>KMAKDSKAPVVEIFDERDGCTSAGSTGKASDAGEKGLLVKVSMQKVGYNAIMAKSVAASYMNK[2x];>[2x]MLDAFSKVITSADGKAAYVGGADLQALKKFVSDGNKRMDAVNAIVSNASCIVSDAVSGMVCENPSLIAPNGGVYSNRKMAACLRDAEIILRYVSYSLLSGDSSVLEDRCLNGLKETYSSLGVPAAGNARAVAIM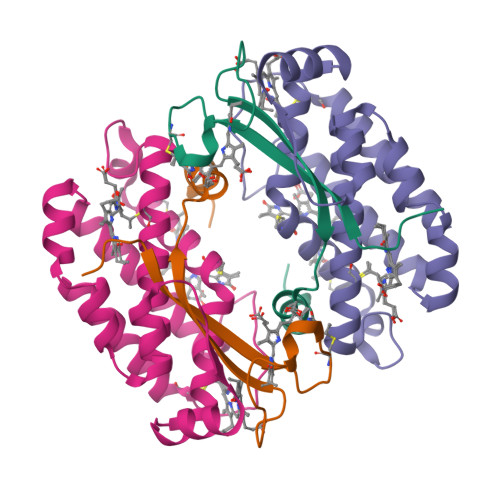KATVNSFINNTAQQKKLSVPSGDCSALASEAGGYFDKVTSAIG> MANKESELNGLDDIHSDIEKLSAHVEKFSDGMDEKYKELTARFDGVKGDNDAIRKAVADATKEYAELSAKHQFFTEELAAMKARLDTPIMRSQAELDDHDRKTAIQLQRNMHEFRGGDPKEFVADESNLVDLKAYRSAVRKMLKVGIESKERVIASMTDVERKAFEASTIGPAFFTPQVLALEVDCNIECASLLDLYGQIEVSRSTFTYMKIADYGQLGEYTCDAKCDAEFGEPGNIRHLEGKTYDYRGVFCFNRKNLQEANYDFLSFMIGAAQRSHRINRNQALMIGKGVNEPKGWLTENCFPVFQTLPVDVNGTSTPAFLAQDWRRFVTSFPAEYGEARSVMHQNVFGYLAAMVDANGRFLFGDGD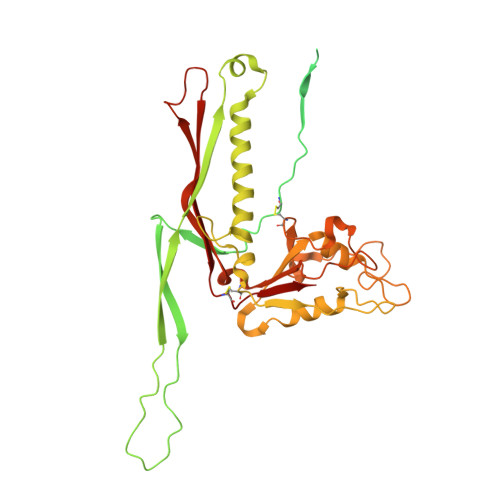LTFTPDLVRERIRISNCLPDPTEGNTKGGTGQDAFAAGSFVAAQAAWKTAFYAVEKRPMFFEQYEGGSSAWCVKYQFGAEDGGFVGCCEHGRILQIG> MIMPQHDQLHRYLFENFAVRGELVTVSETLQQILENHDYPQPVKNVLAELLVATSLLTATLKFDGDITVQLQGDGPMNLAVINGNNNQQMR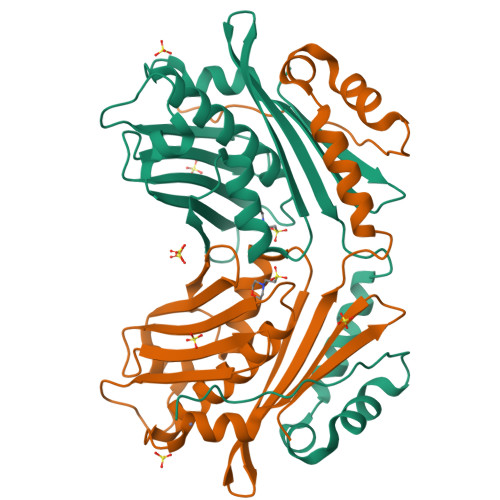GVARVQGEIPENADLKTLVGNGYVVITITPSEGERYQGVVGLEGDTLAACLEDYFMRSEQLPTRLFIRTGDVDGKPAAGGMLLQVMPAQNAQQDDFDHLATLTETIKTEELLTLPANEVLWRLYHEEEVTVYDPQDVEFKCTCSRERCADALKTLPDEEVDSIL6-{[(1R,2S)-2-aminocyclohexyl]amino}-4-[(5,6-dimethylpyridin-2-yl)amino]pyridazine-3-carboxamide | 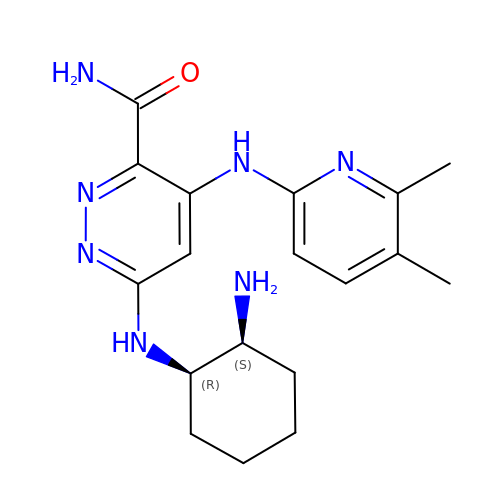C18 H25 N7 O | XJZVCDVZCRLIKN-QWHCGFSZSA-N The T4 replication system centers on a holoenzyme complex that is assembled from the DNA polymerase (gp43) and the sliding clamp (gp45) loaded onto a primer/template junction by the clamp loader complex (gp44/62) in the presence of ATP. The sliding clamp plays a crucial role by encircling the DNA double helix and anchoring the polymerase to the template. Sequence analysis reveals that T4 polymerase contains three main structural regions: an N-terminal domain, a 3′-5′ exonuclease domain responsible for proofreading activity, and a C-terminal polymerase domain. The T4 gp45 sliding clamp forms a trimeric ring structure, with each of the three monomers composed of structurally similar N-terminal and C-terminal domains (NTD and CTD).

To obtain the structure of a one-polymerase complex that more closely aligns with the configuration observed in other B-family polymerase holoenzymes, we strategically disrupted key dimer interface residues. Three mutations (D75R, Q430E, and K432E) were incorporated into the gp43(exo-) polymerase to break two critical salt bridges (Asp75:Arg244 and Lys432:Asp118) and eliminate one hydrogen bond (Gln430:Glu127) within the dimer interface. Following successful expression and purification of this dimer-interface mutant, size exclusion chromatography demonstrated that the complexes assembled with the dimer-interface mutant polymerase exhibited delayed elution compared to those containing the gp43(exo-) polymerase. This elution shift indicated effective disruption of the polymerase dimer interface, yielding T4 holoenzyme complexes with only one polymerase. Cryo-EM analysis provided additional confirmation, with 2D class averages clearly showing the presence of only one polymerase. We subsequently determined the cryo-EM structure of this one-polymerase T4 holoenzyme at an overall resolution of 4.0 Å. A striking feature of this structure is the altered orientation of the sliding clamp, which tilts downward 26° relative to its position in the two-polymerase complex, positioning it perpendicular to the DNA. The primer 3′-terminus occupies the polymerization active site, suggesting an active conformation, although the finger domain remains open in anticipation of an incoming nucleotide binding. This structure thus defines the canonical T4 polymerase holoenzyme architecture, in which a single polymerase associates with the sliding clamp that adopts a largely perpendicular orientation relative to the DNA. The resulting structure shows the clamp positioned perpendicular to the DNA, consistent with other B-family holoenzyme structures. This perpendicular arrangement allows the sliding clamp to move along the DNA on a thin film of water molecules known as the “water skating” mechanism.

> MKEFYISIETVGNNIVERYIDENGKERTREVEYLPTMFRHCKEESKYKDIYGKNCAPQKFPSMKDARDWMKRMERIGLEALGMNDFKLAYISDTYGSEIVYDRKFVRVANCDIEVTGDKFPDPMKAEYEIDAITHYDSIDDRFYVFDLLNSMYGSVSKWDAKLAAKLDCEGGDEVPQEILDRVIYMPFDNERDMLMEYINLWEQKRPAIFTGWNIEGFAVPYIMNRVKMILGERSMKRFSPIGRVKSKLIQNMYGSKEIYSIDGVSILDYLDLYKKFAFTNLPSFSLESVAQHETKKGKLPYDGPINKLRETNHQRYISYNIIDVESVQAIDKIRGFIDLVLSMSYYAKMPFSGVMSPIKTWDAIIFNSLKGEHKVIPQQGSHVKQSFPGAFVFEPKPIARRYIMSFDLTSLYPSIIRQVNISPETIRGEFEVHPIHEYIAGTAPKPSDEYSCSPNGWMYDKHQEGIIPKEIAKVFFQRKDWKKKMFAEEMNAEAIKKIIMKGAGSCSTKPEVERYVKFSDDFLNELSNYTESVLNSLIEECEKAATLANTNQLNRKILINSLYGALGNIHFRYYDLRNATAITIFGQVGIQWIARKINEYLNKVCGTNDEDFIAAGDTDSVYVCVDKVIEKVGLDRFKEQNDLVEFMNQFGKKKMEPMIDVAYRELCDYMNNREHLMHMDREAISCPPLGSKGVGGFWKAKKRYALNVYDMEDKRFAEPHLKIMGMETQQSSTPKAVQEALEESIRRILQEGEESVQEYYKNFEKEYRQLDYKVIAEVKTANDIAKYDDKGWPGFKCPFHIRGVLTYRRAVSGLGVAPILDGNKVMVLPLREGNPFGDKCIAWPSGTELPKEIRSDVLSWIDHSTLFQKSFVKPLAGMCESAGMDYEEKASLDFLFG;>[3x]MKLSKDTTALLKNFATINSGIMLKSGQFIMTRAVNGTTYAEANISDVIDFDVAIYDLNGFLGILSLVNDDAEISQSEDGNIKIADARSTIFWPAADPSTVVAPNKPIPFPVASAVTEIKAEDLQQLLRVSRGLQIDTIAITVKEGKIVINGFNKVEDSALTRVKYSLTLGDYDGENTFNFIINMANMKMQPGNYKLLLWAKGKQGAAKFEGEHANYVVALEADSTHDF> MAFLRSMWGVLSALGRSGAELCTGCGSRLRSPFSFVYLPRWFSSVLASSPKKPVSSYLRFSKEQLPIFKAQNPDAKTTELIRRIAQRWRELPDSKKKIYQDAYRAEWQVYKEEISRFKEQLTPSQIMSLEKEIMDKHLKRKAMTKKKELTLLGKPKRPRSAYNVYVAERFQEAKGDSPQEKLKTVKENWKNLSDSEKELY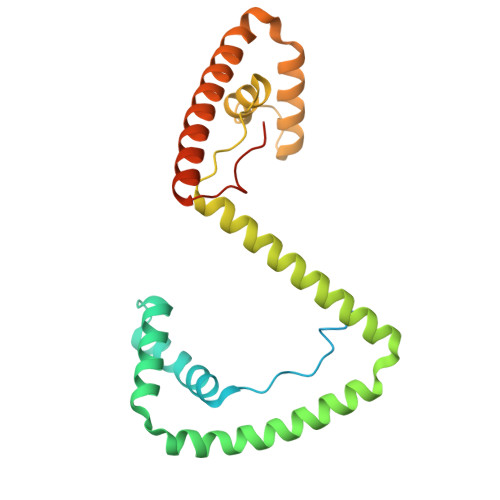IQHAKEDETRYHNEMKSWEEQMIEVGRKDLLRRTIKKQRKYGAEEC> MHHHHHHATSSPS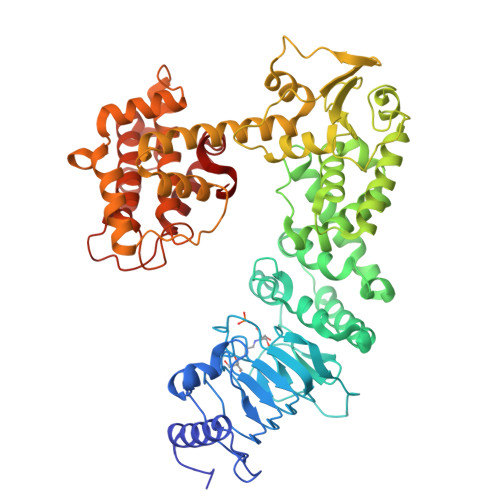SPADWAKKLTDAVLRQKAGETLTAADRDFSNADFRNITFSKILPPSFMERDGDIIKGFNFSNSKFTYSDISHLHFDECRFTYSTLSDVVCSNTKFSNSDMNEVFLQYSITTQQQPSFIDTTLKNTLIRHKANLSGVILNEPDNSSPPSVSGGGNFIRLGDIWLQMPLLWTENAVDGFLNHEHNNGKSILMTIDSLPDKYSQEKVQAMEDLVKSLRGGRLTEACIRPVESSLVSVLAHPPYTQSALISEWLGPVQERFFAHQCQTYNDVPLPAPDTYYQQRILPVLLDSFDRNSAAMTTHSGLFNQVILHCMTGVDCTDGTRQKAAALYEQYLAHPAVSPHIHNGLFGNYDGSPDWTTRAADNFLLLSSQDSDTAMMLSTDTLLTMLNPTPDTAWDNFYLLRAGENVSTAQISPVELFRHDFPVFLAAFNQQATQRRFGELIDIILSTEEHGELNQQFLAATNQKHSTVKLIDDASVSRLATIFDPLLPEGKLSPAHYQHILSAYHLTDATPQKQAETLFCLSTAFARYSSSAIFGTEHDSPPALRGYAEALMQKAWELSPAIFPSSEQFTEWSDRFHGLHGAFTCTSVVADSMQRHARKYFPSVLSSILPLAWA> MWKRSEQMKIKSGKCNMAAAMETEQLGVEIFETADCEENIESQDRPKLEPFYVERYSWSQLKKLLADTRKYHGYMMAKAPHDFMFVKRNDPDGPHSDRIYYLAMSGENRENTLFYSEIPKTINRAAVLMLSWKPLLDLFQATLDYGMYSREEELLRERKRIGTVGIASYDYHQGSGTFLFQAGSGIYHVKDGGPQGFTQQPLRPNLVETSCPNIRMDPKLCPADPDWIAFIHSNDIWISNIVTREERRLTYVHNELANMEEDARSAGVATFVLQEEFDRYSGYWWCPKAETTPSGGKILRILYEENDESEVEIIHVTSPMLETRRADSFRYPKTGTANPKVTFKMSEIMIDAEGRIIDVIDKELIQPFEILFEGVEYIARAGWTPEGKYAWSILLDRSQTRLQIVLISPELFIPVEDDVMERQRLIESVPDSVTPLIIYEETTDIWINIHDIFHVFPQSHEEEIEFIFASECKTGFRHLYKITSILKESKYKRSSGGLPAPSDFKCPIKEEIAITSGEWEVLGRHGSNIQVDEVRRLVYFEGTKDSPLEHHLYVVSYVNPGEVTRLTDRGYSHSCCISQHCDFFISKYSNQKNPHCVSLYKLSSPEDDPTCKTKEFWATILDSAGPLPDYTPPEIFSFESTTGFTLYGMLYKPHDLQPGKKYPTVLFIYGGPQVQLVNNRFK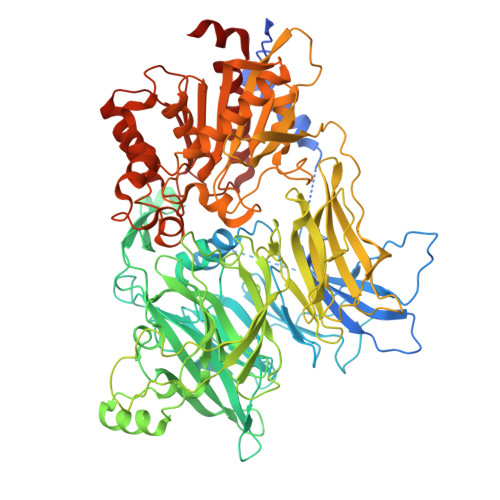GVKYFRLNTLASLGYVVVVIDNRGSCHRGLKFEGAFKYKMGQIEIDDQVEGLQYLASRYDFIDLDRVGIHGWSYGGYLSLMALMQRSDIFRVAIAGAPVTLWIFYDTGYTERYMGHPDQNEQGYYLGSVAMQAEKFPSEPNRLLLLHGFLDENVHFAHTSILLSFLVRAGKPYDLQIYPQERHSIRVPESGEHYELHLLHYLQENLGSRIAALKVI>MANVNKTPGKTRRAEVAGGGFAGLTAAIALKQNGWDVRLHEKSSELRAFGAGIYLWHNGLRVLEGLGALDDVLQGSHTPPTYETWMHNKSVSKETFNGLPWRIMTRSHLHDALVNRARALGVDISVNSEAVAADPVGRLTLQTGEVLEADLIVGADGVGSKVRDSIGFKQDRWVSKDGLIRLIVPRMKKELGHGEWDNTIDMWNFWPRVQRILYSPCNENELYLGLMAPAADPRGSSVPIDLEVWVEMFPFLEPCLIEAAKLKTARYDKYETTKLDSWTRGKVALVGDAAHAMAPALAQGAGCAMVNAFSLSQDLEEGSSVEDALVAWETRIRPITDRCQALSGDYAANRSLSKGNMFTPAALEAARYDPLRRVYS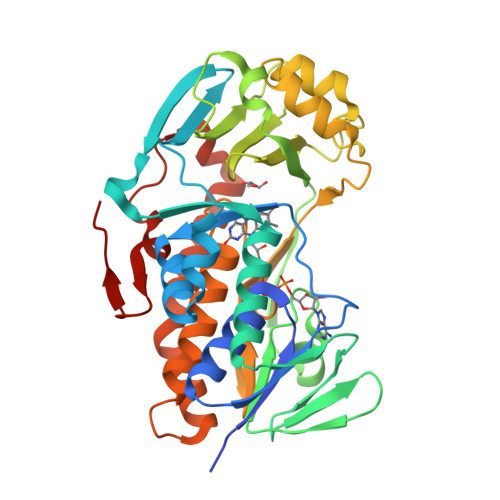WPQ[2x]> LGRLVSPGPCPRPYLVITEQPKQRGMRFRYECEGRSAGSILGESSTEASKTQPAIELRDCGGLREVEVTACLVWKDWPHRVHPHSLVGKDCTDGVCRVRLRPHVSPRHSFNNLGIQCVRKKEIEAAIERKIQLGIDPYNAGSLKNHQEVDMNVVRICFQASYRDQQGHLHRMDPILSEPVYDKKSTNTSELRICRINKESGPCTGGEELYLLCDKVQKEDISVVFSTASWEGRADFSQADVHRQIAIVFKTPPYEDLEISEPVTVNVFLQ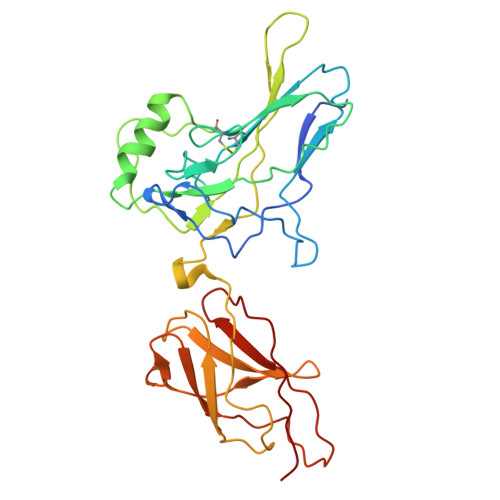RLTDGVCSEPLPFTYLPR> GSGPVKPIQEAVSELMEIEASGTDDDDGSIDEALVTVYEEIESADGNITGVPSGFTELDRMTY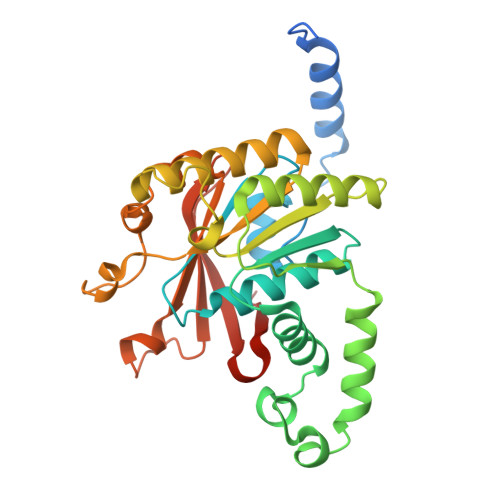GYKRRNFVLIAARPSMGKTAFALKQAKNMSDNDDVVNLHSLEMGKKENIKRLIVTAGSINAQKIKAARRDFASEDWGKLSMAIGEISNSNINIFDKAGQSVNYIWSKTRQTKRKNPGKRVIVMIDYLQLLEPAKANDSRTNQISQISRDLKKMARELDVVVIALSQLSRQVEQRQDKRPMLSDLRESGQLEQDADIIEFLYRDDYYDKESESKNIVEVIIAKHRDGPVGTVSLAFIKEYGNFVNLERRFDDR For promoter-specific transcription, RNAP and general transcription factors (GTFs) are recruited to the promoter DNA to form the pre−initiation complex (PIC). In this study, we determined the X-ray structure of TFEα and the cryo-EM structures of three forms of archaeal RNAP, including the apo-form, RNAP–TFEα binary complex, and RNAP–TFEα–DNA ternary complex. The structures reveal that direct binding of TFEα can shift the clamp conformation from a closed conformation to an open conformation. Our results support the universally conserved mechanisms of transcription initiation in all three domains of life by showing that direct binding of TFEα, a conserved GTF in archaeal-eukaryal RNAP systems, can open the clamp of the stalk-containing RNAPs.

After screening derivatives of TFEα, we found that the 13 kDa fragment Pfu TFEα (TFEαΔZRD, 1–110 amino acid residues) was crystallized. The structure was solved by a single wavelength anomalous dispersion (SAD) at 3.2 Å and the resolution of the structure was improved to 2.6 Å with a native crystal. There were eight molecules in the asymmetric unit of the SAD structure and two molecules in the asymmetric unit of the native structure. The TFEαΔZRD structure consists of the N-terminal eWHD (residues 5–86) and a long α-helix (α5) that connects the eWHD and the ZRD. Superposition of the globular part of the eWHD from the 10 crystallographically independent structures (average root-mean-square deviation in α-carbon positions are 0.369–0.589 Å over residues 8–62) reveal flexibilities in the wing and the α5 linker. The conformation of the wing can change about 24° (~13 Å), and the α5 can be bent at ~21° (~12 Å) for the eWHD. These results show a potential structural adaptability of TFEα during the transcription initiation process.

>MGRDKKNTALLDMARDIGGDEAVEVVKALEKKGEATDEELAELTGVRVNTVRKMLYALYDAKLATMRRVRDDETGWYYYYWRIDTKRLPEVIRTRKLQELEKLKQMLQEE[8x]> MATLTAKNLAKA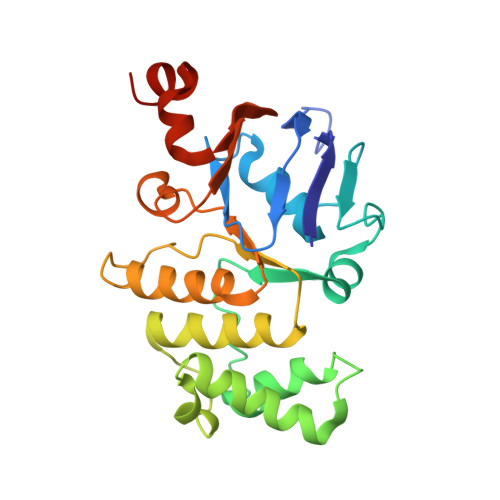YKGRRVVEDVSLTVNSGEIVGLLGPNGAGKTTTFYMVVGIVPRDAGNIIIDDEDISLLPLHARARRGIGYLPQEASIFRRLSVYDNLMAVLQIRDDLTSEQREDRAKELMEEFHIEHLRDSLGQALSGGERRRVEIARALAANPKFILLDEPFAGVDPISVIDIKRIIEHLRDSGLGVLITDHNVRETLAVCERAYIVSQGHLIAHGTPQQILEDEQVKRVYLGEDFRL> GPGHMEASPASGPRHLMDPHIFTSNFNNGIGRHKTYLCYEVERLDNGTSVKMDQHRGFLHNQAKNLLCGFYGRHAALRFLDLVPSLQLDPAQIYRVTWFISWSPCFSWGCAGEVRAFLQENTHV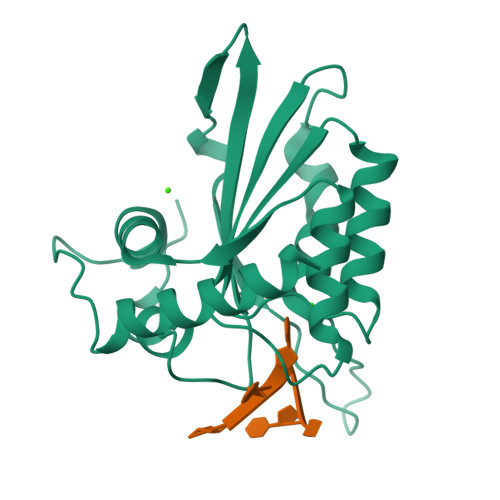RLRIFAARIYDYDPLYKEALQMLRDAGAQVSIMTYDEFKHCWDTFVDHQGAPFQPWDGLDEHSQALSGRLRAILQNQGN>[2x]MRVGLVGWRGMVGSVLMQRMVEERDFDLIEPVFFS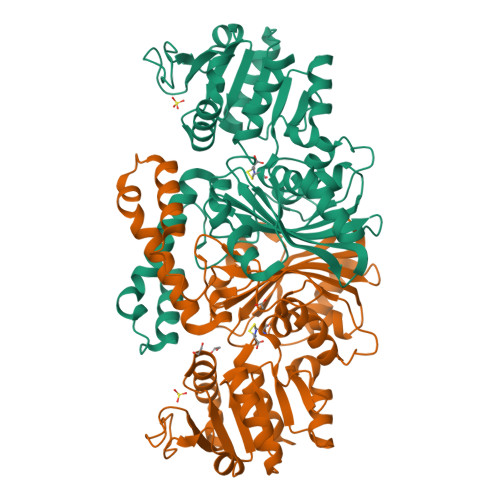TSQIGVPAPNFGKDAGMLHDAFDIESLKQLDAVITCQGGSYTEKVYPALRQAGWKGYWIDAASTLRMDKEAIITLDPVNLKQILHGIHHGTKTFVGGNCTVSLMLMALGGLYERGLVEWMSAMTYQAASGAGAQNMRELISQMGVINDAVSSELANPASSILDIDKKVAETMRSGSFPTDNFGVPLAGSLIPWIDVKRDNGQSKEEWKAGVEANKILGLQDSPVPIDGTCVRIGAMRCHSQALTIKLKQNIPLDEIEEMIATHNDWVKVIPNERDITARELTPAKVTGTLSVPVGRLRKMAMGDDFLNAFTVGDQLLWGAAEPLRRTLRIILAEK>GGSHDCAKVDLENAELRRKLIRTKRAFEDTYEKLRMANKAKAQVEKDIKNQILKTHNVLRNVRSNMENEL[4x]

In flies, Centrosomin (Cnn) forms a phosphorylation-dependent scaffold that recruits proteins to the mitotic centrosome, but how Cnn assembles into a scaffold is unclear. We show that scaffold assembly requires conserved leucine zipper (LZ) and Cnn-motif 2 (CM2) domains that co-assemble into a 2:2 complex in vitro. Purified CM2 forms a stable 2:2 tetramer with the purified LZ of the PReM domain, and we solve the crystal structure of the LZ:CM2 complex, revealing that helical dimers of LZ and CM2 interact in an anti-parallel fashion. Thus, Cnn molecules have an intrinsic ability to form large, LZ:CM2-interaction-dependent assemblies that are critical for mitotic centrosome assembly.

SEC-MALS analysis revealed that LZ formed a stable homo-tetramer in solution, while CM2 behaved as a stable homo-dimer. Intriguingly, although CM2 showed no tendency to tetramerise in solution, apo-CM2 crystals contained two copies of the CM2 homo-dimer that interacted in an anti-parallel fashion to form a homo-tetramer. A splayed C terminus was also observed in crystals of CM2 alone, indicating it is a feature of the CM2 sequence rather than being driven by the interaction with the LZ. Zn2+ was not included in our protein preparations, so it must have been incorporated into the dimer in the bacteria and then retained throughout the purification process, indicating tight binding. Addition of EDTA to WT CM2, or mutation of the Zn2+-coordinating His and Cys residues to Ala (CM2-HCAA), prevented dimerization in vitro, confirming that Zn2+ plays a structural role within CM2. The HCAA mutation perturbed Cnn-scaffold assembly in vivo, although not to the same extent as deleting the entire CM2 domain, suggesting that Zn2+ binding enhances scaffold assembly in vivo but is not essential.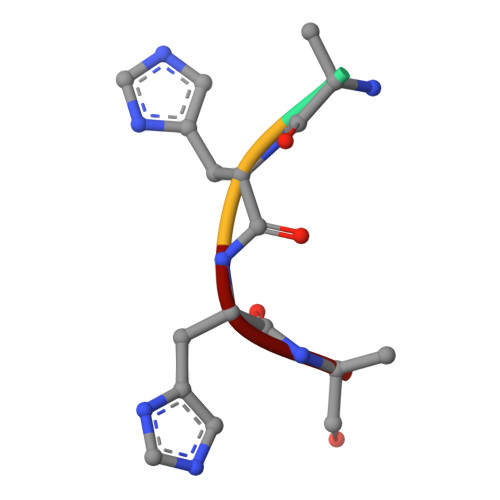> AHHA>[2x]SRTI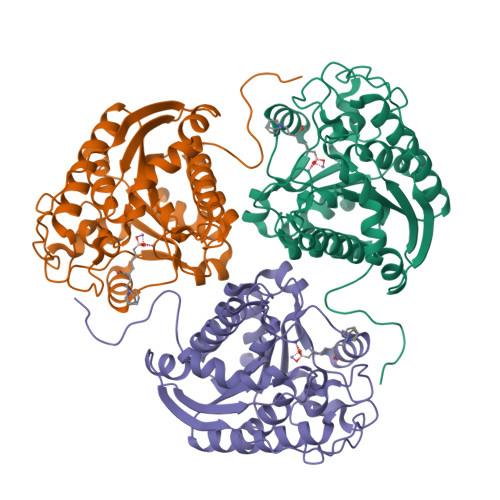GIIGAPFSKGQPRGGVEEGPTVLRKAGLLEKLKEQECDVKDYGDLPFADIPNDSPFQIVKNPRSVGKASEQLAGKVAEVKKNGRISLVLGGDHSLAIGSISGHARVHPDLGVIWVDAHTDINTPLTTTSGNLHGQPVSFLLKELKGKIPDVPGFSWVTPCISAKDIVYIGLRDVDPGEHYILKTLGIKYFSMTEVDRLGIGKVMEETLSYLLGRKKRPIHLSFDVDGLDPSFTPATGTPVVGGLTYREGLYITEEIYKTGLLSGLDIMEVNPSLGKTPEEVTRTVNTAVAITLACFGLAREGNHKPIDYL> GUGUGCCCGGCAUGGGUGCAGUCUAUAGGGUGAGAGUCCCGAACUGUGAAGGCAGAAGUAACAGUUAGCCUAACGCAAGGGUGUCCGUGGCGACAUGGAAUCUGAAGGAAGCGGACGGCAAACCUUCGGUCUGAGGAACAC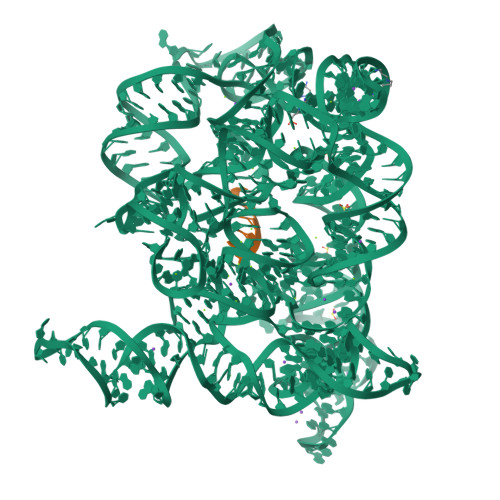GAACUUCAUAUGAGGCUAGGUAUCAAUGGAUGAGUUUGCAUAACAAAACAAAGUCCUUUCUGCCAAAGUUGGUACAGAGUAAAUGAAGCAGAUUGAUGAAGGGAAAGACUGCAUUCUUACCCGGGGAGGUCUGGAAACAGAAGUCAGCAGAAGUCAUAGUACCCUGUUCGCAGGGGAAGGACGGAACAAGUAUGGCGUUCGCGCCUAAGCUUGAACCGCCGUAUACCGAACGGUACGUACGGUGGUGUG;> GGGGUUAU>MPVFTASFQCVTLFGQPASAADAQPLLQGQRPFLHLHARRRRPCGPMLISKSPPYPASEETREWEADGQHEHTDELRETTTTMIDGIRTALRSIGEGEISISAYDTSLVALLKRLDGGDGPQFPSTIDWIVQNQLPDGSWGDASFFMMGDRIMSTLACVVALKSWNIHTDKCERGLLFIQENMWRLAHEEEDWMLVGFEIALPSLLDMAKDLDLDIPYDEPALKAIYAERERKLAKIPRDVLHSMPTTLLHSLEGMVDLDWEKLLKLRCLDGSFHCSPASTATAFQQTGDQKCFEYLDGIVKKFNGGVPCIYPLDVYERLWAVDRLTRLGISRHFTSEIEDCLDYIFRNWTPDGLAHTKNCPVKDIDDTAMGFRLLRLYGYQVDPCVLKKFEKDGKFFCLHGESNPSSVTPMYNTYRASQLKFPGDDGVLGRAEVFCRSFLQDRRGSNRMKDKWAIAKDIPGEVEYAMDYPWKASLPRIETRLYLDQYGGSGDVWIGKVLHRMTLFCNDLYLKAAKADFSNFQKECRVELNGLRRWYLRSNLEKFGGTDPQTTLMTSYFLASANIFEANRAAERLGWARVALLADAVSSHFRRIGGPKNSTSNLEELISLVPFDDAYSGSLREAWKQWLMAWTAKESSQESIEGDTAILLVRAIEIFGGRHVLTGQRPDLWEYSQLEQLTSSICCKLSRRVLAQENGESTEKVEEIDQQ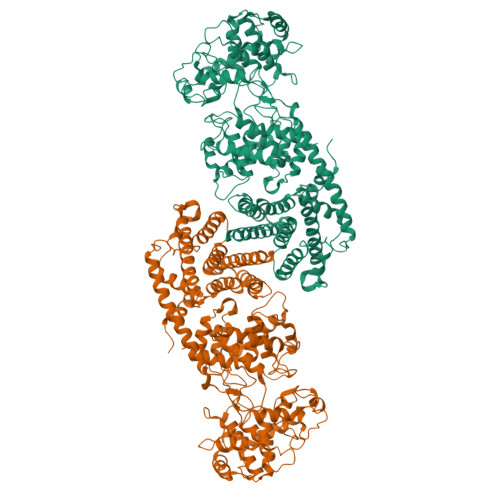VDLEMQELTRRVLQGCSAINRLTRETFLHVVKSFCYVAYCSPETIDSHIDKVIFQDVIEFHHHHHH[2x]CYTARABINE 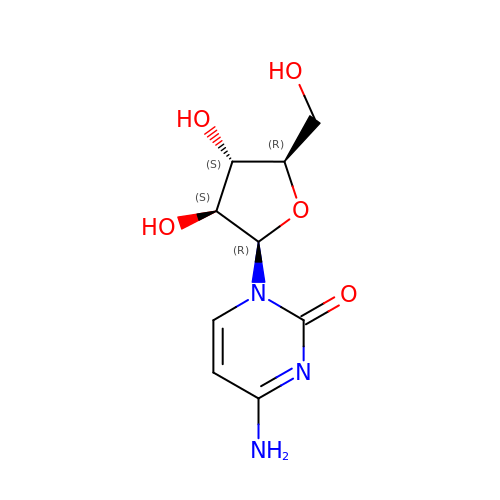| C9 H13 N3 O5 | UHDGCWIWMRVCDJ-CCXZUQQUSA-N> GMSKNERDTSFNKNGCLVFVSRLWDLDKLGMFHHPVSAEELPDYHTVIKRPVDLSSIRDGIEKGTYATDVD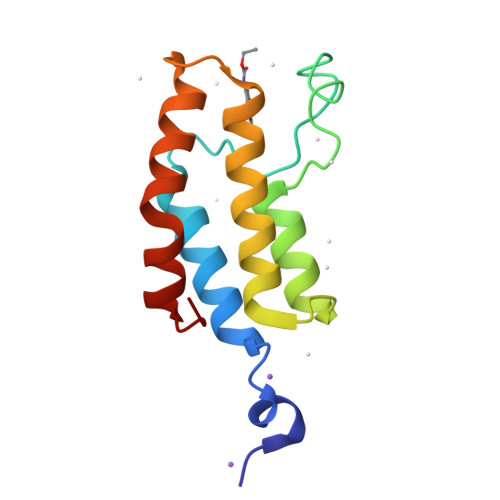VQNDVARMITNALEYNAKGSTWYQEAMSFRKTYLDLARQSGLVVD>[4x]MGSDKIHHHHHHMQARWIGNMMFHVRTDSNHDVLMDTKEEVGGKDAAPRPLELVLTGLMGCTGMDVVSILRKMKVIDQMKDFR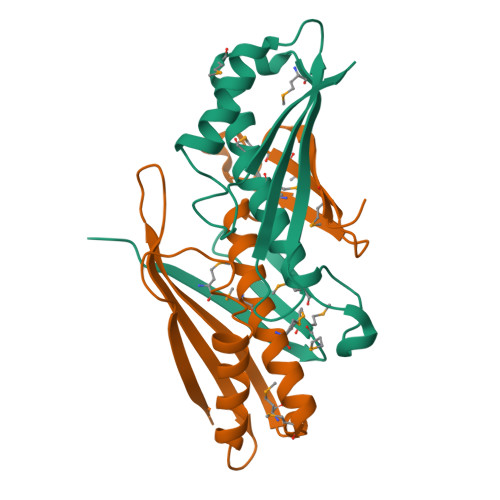IEIEYERTEEHPRIFTKVHLKYIFKFDGEPPKDKVEKAVQLSQEKYCSVSAILKCSSKVTYEIVYEN ethyl 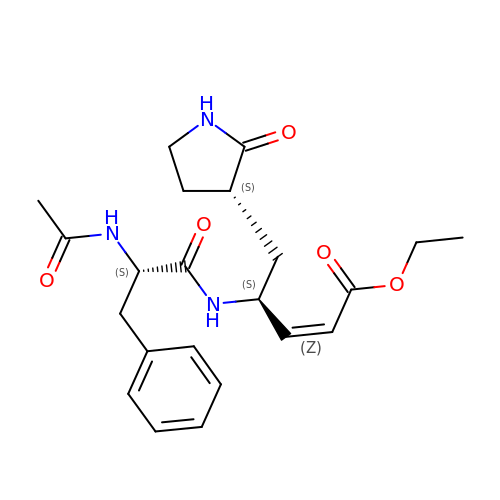(2Z,4S)-4-[(N-acetyl-L-phenylalanyl)amino]-5-[(3S)-2-oxopyrrolidin-3-yl]pent-2-enoate | C22 H29 N3 O5 | YYPCDXRHVHVVTA-OTWHNJEPSA-N>[4x]GPTAAALERLTTEEVQGLSDVKTLVNQLYEALNVREHQLQKEVELTTQLETLQQELLPLEEKKLELEQVANRRSNWMAWAGLGLMSVQFGILARLTWWEYSWDIMEPVTYFVTYGTAMAAYAYFVLTREEYILNDVRDRQQLLLLHKKAKKTGFDVNQYNVLKDQIAKLELDLKRLRDPLKLRLPPKAAAKEEGGWSHPQFEK;>[3x]GPTAAALETAVYSKSGGLLPEPHRTSFGIIRLILTVVPGLLIGAAISKNIANFLEENDLFVPSDDDDDDD;> GPTAAALEPHPEEKKKKRSGFRDRKVMEYENRIRAYSTPDKIFRYFATLKVISEPGEAEVFMTPEDFVRSITPNEKQPEHLGLDQYIIKRFDGKKISQEREKFADEGSIFYTLGECGLISFSDYIFLTTVLSTPQRNFEIAFKMFDLNGDGEVDMEEFEQVQSIIRSQTSMGMRHRDRPTTGNTLKSGLCSALTTYFFGADLKGKLTIKNFLEFQRKLQHDVLKLEFERHDPVDGRITERQFGGMLLAYSGVQSKKLTAMQRQLKKHFKEGKGLTFQEVENFFTFLKNINDVDTALSFYHMAGASLDKVTMQQVARTVAKVELSDHVCDVVFALFDCDGNGELSNKEFVSIMKQRLMRGLEKPKDMGFTRLMQAMWKCAQETAWDFALPKQSNW;> HHSRVSVAARDGSFTVSAQKNVEHGIIYIGKPSLRKQRFMQFSSLEHEGEYYMTPRDFLFSVMFEQMERKTSVKKLTKKDIEDTLSGIQTAGCGSTFFRDLGDKGLISYTEYLFLLTILTKPHSGFHVAFKMLDTDGNEMIEKREFFKLQKIISKQDDLMTVKTNETGYQEAIVKEPEINTTLQMRFFGKRGQRKLHYKEFRRFMENLQTEIQEMEFL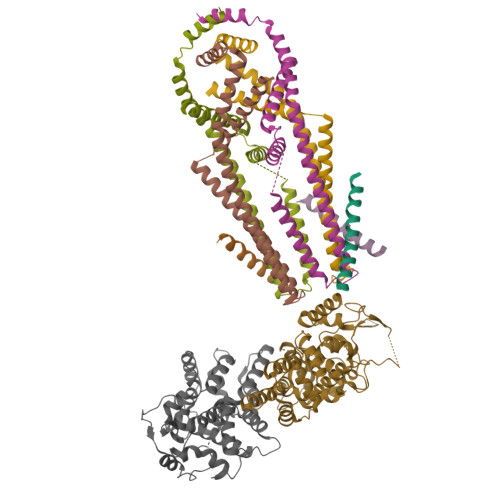QFSKGLSFMRKEDFAEWLLFFTNTENKDIYWKNVREKLSAGESISLDEFKSFCHFTTHLEDFAIAMQMFSLAHRPVRLAEFKRAVKVATGQELSNNILDTVFKIFDLDGDECLSHEEFLGVLKNRMHRGLWVPQHQSIQEYWKCVKKESIKGVKEVWKQAGKGLF> AAIVKLGGDDGSLAFVPNNITVGAGESIEFINNAGFPHNIVFDEDAVPAGVDADAISAEDYLNSKGQTVVRKLTTPGTYGVYCD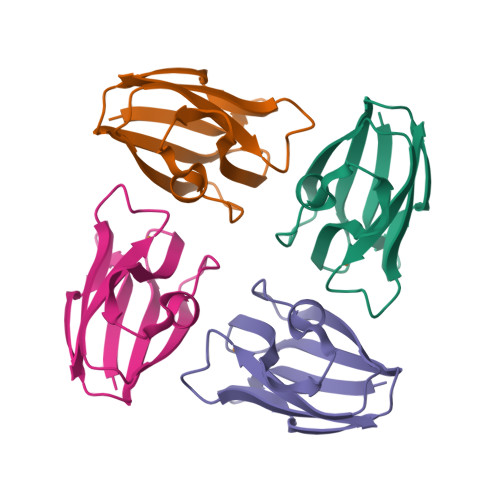PHSGAGMKMTITVQ>[4x]MIWKRKITLEALNAMGEGNMVGFLDIRFEHIGDDTLEATMPVDSRTKQPFGLLHGGASV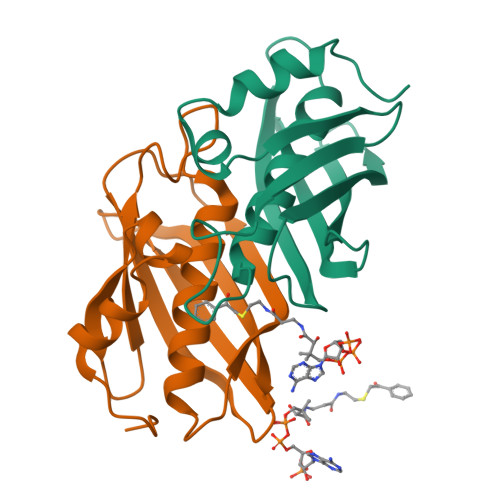VLAESIGSVAGYLCTEGEQKVVGLEINANHVRSAREGRVRGVCKPLHLGSRHQVWQIEIFDEKGRLCCSSRLTTAIL Sco GlgEI is a homolog of Mycobacteria tuberculosis (Mtb) GlgE. In Mtb, GlgE is part of a biosynthetic pathway that generates α-glucans from trehalose and is a genetically validated anti-TB target. GlgE enzymes polymerize maltose-1-phosphate (M1P) to linear α-(1→4) glucans, Figure 3A. In these studies, we used Sco GlgEI-V279S, which possesses the same active site topology and active site residues as Mtb GlgE; however, Sco GlgEI-V279S is more stable and is highly amenable to structural studies.

While compounds 11–13 did not inhibit Sco GlgEI-V279S at the concentrations evaluated, an X-ray crystal structure of the Sco GlgE1-V279S/13 complex was solved to a resolution of 2.73 Å. The Sco GlgEI-V279S/13 complex structure was resolved to a resolution of 2.73 Å, and the 2Fo-Fc composite omit map illustrated the presence of compound 13 in the M1P binding site of Sco GlgEI-V279S. The difference density maps show strong density for the glucose moiety in the -2 subsite and the carbocycle in the −1 subsite. However, the cyclohexyl moiety of compound 13 exhibits only weak difference density suggesting a lack of sufficient binding interactions with the residues forming the Sco GlgEI-V279S +1 site. Inspection of the −1 subsite illustrates that the carbocycle C(3)-OH and C(7)-OH functional groups are in an axial conformational and form a bidentate hydrogen-bonded interaction with the side chain oxygen atoms of the Asp 394 nucleophile. Since both Sco GlgEI-V279S/AGV and Sco GlgEi-V279S/13 crystals were formed at pH 7.5 and due to the proximity of the secondary amine of compound 13 with the side chain of Glu 423, it is hypothesized that the nitrogen atom of compound 13 is protonated and harbors a positive charge as anticipated for the primary ammonium moiety in AGV. Therefore, the 3.2 Å distant interaction between Glu 423 and the amine of 13 should be considered an ionic interaction. Unfortunately, the compound 13 carbocycle interactions with the Glu 423 (general acid/base) were weakened by addition of the cyclohexyl moiety due to steric hindrance. This also promotes bond rotation in the Asp 394 side chain, which weakens an otherwise strong bidentate hydrogen-bonded interaction between Asp 394 and hydroxyls 2 and 7 of compound 13. Unfortunately, these minor disruptions in binding lack compensating interactions between the +1 subsite and the cyclohexyl moiety of 13, which appears to form only transitory interactions with side chains of the +1 subside.

>MPATHHSSATSAERPTVVGRIPVLDVRPVVQRGRRPAKAVTGESFEVSATVFREGHDAVGANVVLRDPRGRPGPWTPMRELAPGTDRWGATVTAGETGTWSYTVEAWGDPVTTWRHHARIKIPAGLDTDLVLEEGARLYERAAADVPGREDRRELLAAVDALRDESRPAASRLAAALTPQVDAVLARHPLRDLVTSSDPLPLLVERERALYGAWYEFFPRSEGTPHTPHGTFRTAARRLPAIAAMGFDVVYLPPIHPIGTTHRKGRNNTLSATGDDVGSPWAIGSPEGGHDSIHPALGTLDDFDHFVTEAGKLGLEIALDFALQCSPDHPWVHKHPEWFHHRPDGTIAHAENPPKKYQDIYPIAFDADPDGLATETVRILRHWMDHGVRIFRVDNPHTKPVAFWERVIADINGTDPDVIFLAEAFTRPAMMATLAQIGFQQSYTYFTWRNTKQELTEYLTELSGEAASYMRPNFFANTPDILHAYLQHGGRPAFEVRAVLAATLSPTWGIYSGYELCENTPLREGSEEYLDSEKYQLKPRDWTRAAREGTTIAPLVTRLNTIRRENPALRQLRDLHFHPTDKEEVIAYSKRQGSNTVLVVVNLDPRHTQEATVSLDMPQLGLDWHESVPVRDELTGETYHWGRANYVRLEPGRTPAHVCTVLRPSHPQIGGSHTTALHHHHHH[2x]Spliceosomal proteins Hsh49p and Cus1p are components of SF3b, which together with SF3a, Msl1p/Lea1p, Sm proteins, and U2 snRNA, form U2 snRNP, which plays a crucial role in pre-mRNA splicing. Hsh49p, comprising two RRMs, forms a heterodimer with Cus1p. The structures show that the Cus1 fragment binds to the α-helical surface of Hsh49p RRM1, opposite the four-stranded β-sheet, leaving the canonical RNA-binding surface available to bind RNA. Hsh49p binds the 5′ end region of U2 snRNA via RRM1.

The Hsh49p–Cus1(290–368)p construct yielded small needle-like trigonal crystals, which diffracted to a maximum resolution of 2.7 Å, but at this point we were unable to solve the structure by molecular replacement or isomorphous replacement, partly due to twinning. It was previously shown that RRM1 of Hsh49p binds to Cus1p, so we coexpressed RRM1 of Hsh49p with the same Cus1p peptide (290–368). All four molecules in the asymmetric unit are very similar with average overall RMSDs for the main chain of 0.22 Å for RRM1 and 0.42 Å for Cus1(290–368)p. The higher resolution crystal structure of RRM1–Cus1(290–368)p was used for the detailed analysis of the structure of Cus1(290–368)p and the interface between RRM1 and Cus1(290–368)p. The Cus1(290–368) domain is folded with most secondary structure elements located at its periphery, and it covers almost the entire α-helical side of RRM1. An extensive interface is created between Cus1(290–368)p and the α-helical surface of RRM1 of Hsh49p. At the center of this interaction surface, a completely conserved tryptophan (Trp312), located at the bottom of α2 of Cus1(290–368)p, lies flat in a hydrophobic cleft on the surface of RRM1 created by α1, α2, and the extended linker between α2 and β4. The interface between RRM1 and Cus1(290–368)p is stabilized by face-to-face hydrophobic stacking interactions. The buried surface area of the interface is about 960 Å2 with a complex formation significance score of one, implying that this interface plays an essential role in complex formation (PDBe PISA [Krissinel and Henrick 2007]). The Hsh49p RRM1–Cus1(290-368)p structure fits well into cryo-EM density of the Bact spliceosome, corroborating the biological relevance of our crystal structure.

>[4x]GGSNYSADSGNTVYVGNIDPRITKEQLYELFIQINPVLRIKYPKDKVLQAYQGYAFIEFYNQGDAQYAIKIMNNTVRLYDRLIKVRQVTNSTGTTNLPSNIS;>MAVGSRPGRISQELRAIMNLPEGQLPPWCMKMKDIGLPTGYPDLKIAGLNWDITNLKGDVYGKIIPNHHSRSKKQGRNYFGALI[4x]>MTDNKRPQLKDKEPAAKPARTRKPKNETVALVVEATTEAEAKKSLREGGLVPAAHEIMIPVGNMILAVDTQVLDKCALALAASDDPGRWFAENESLIHSTVFAPVAKGLHRVYPLLSVRPEVPAGYEASWPTQDHMPGLHLVVGGTGAGKSSYLASQDLTLVIRWGEPAERFDVEGATHAVSDLNEALAVAFVMARAGYRPAIDSFRNLVFGIESAAGEGGISTALYSAMTAINNVCSRLGIVVMVVVNPMATEAKAELVYNNMAASVAGMTVLMDGAVSKQTVRTLSGRTWGVGKQPKAAVTEEVIPRATVVPQPSA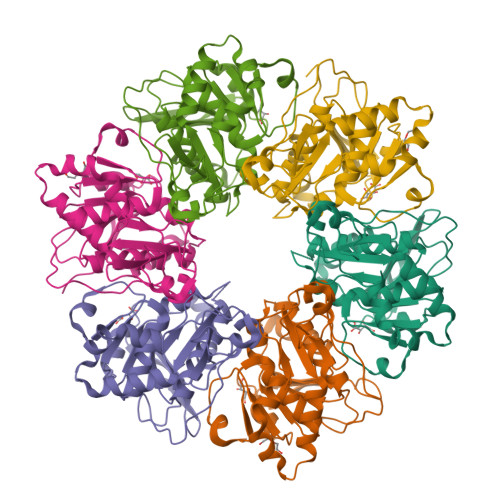VVRNTRLESQTIDVSDDDLNNEPGRQGSRKHI[8x]> GSGGPSATTPPPPTYSELQITRIQDYLRDIE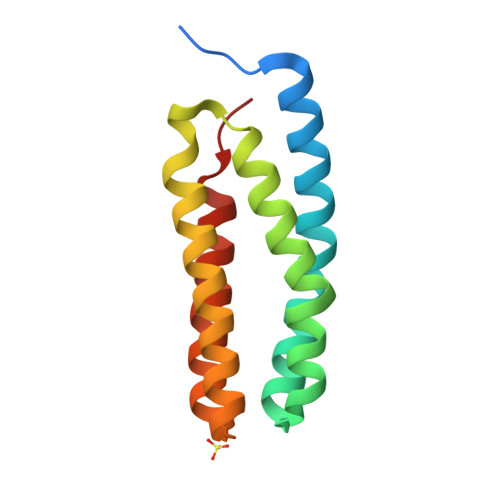KNAERFADLEVSVAKGDWQEARNIMRGPLGEMLMDMRALNRNLLAKDQPTPTALTRALTDDFLKIDQGADLDSVTVAQEGFREAEADFKAYLNSLPELS>HTDLSGKVFVFPRESVTDHVNLITPLEKPLQNFTLCFRAYSDLSRAYSLFSYNTQGRDNELLVYKERVGEYSLYIGRHKVTSKVIEKFPAPVHICVSWESSSGIAEFWINGTPLVKKGLRQGYFVEAQPKIVLGQEQDSYGGKFDRSQSFVGEIGDLYMWDSVLPPENILSAYQGTPLPANILDWQALNYEIRGYVIIKPLVWV[5x]

Serum amyloid P component (SAP) is a normal plasma glycoprotein that recognizes and binds to amyloid fibres in a calcium-dependent fashion wherever these are deposited in tissues. In summary, the structure of SAP is comprised of five identical 204-residue subunits associated in a ring 95 Å in diameter and 35 Å deep, with radial symmetry creating a central pore 20 Å wide. Each protomer consists of 15 β-strands (labelled A to O from the N-terminus to the C-terminus) arranged in two large β-sheets in the form of a flattened β-barrel with jelly-roll topology. The β-sheets are held nearly perpendicular to the radial symmetry, creating two separate and distinct faces: the A face, which contains five α-helices, and the opposing B face, which contains five double metal-binding sites formed by the coordination of six localized protein residues.

We also report a high-resolution analysis of the interaction of N-acetyl-d-proline, a substructure of CPHPC, with SAP in comparison with the l-isomer. Crystals of the SAP–N-acetyl-d-proline complex grew with a 45-fold molar excess of N-acetyl-d-proline in 60 mM Tris–HCl pH 8.0, 10 mM CaCl2, 84 mM NaCl, 20%(v/v) glycerol, 17%(v/v) PEG 550 MME. The molecular-replacement solution showed one SAP pentamer in the asymmetric unit and an estimated solvent content of 53%. Five d-proline ligands were observed bound to each SAP pentamer via the double calcium sites on each subunit. The puckered proline ring plane is parallel to that of Tyr74, but the penetration of the ligand into the pocket is not sufficiently deep to achieve stacking of all atoms. Rather, the proline Cγ and Cδ atoms interact with Tyr64, Cβ and Cγ interact with Tyr74 and Cβ interacts with Leu62. The proline NH is 4.2 Å away from Tyr74 OH. The peptide plane has been built as cis; this was a marginal decision based on the proximity of hydrogen-bond partners (the side-chain amide of Gln148 at 3.9 Å and the hydroxyls of Tyr64 at 4.6 Å and of Tyr74 at 5.5 Å). One molecule of glycerol was observed binding close to Pro29 on each subunit. d values show a 2000-fold increase in the apparent affinity for binding of half of the double-headed CPHPC compound by the SAP subunit: 8.8 nM compared with 18.6 µM for N-acetyl-d-proline and 322 µM for N-acetyl-l-proline.6-(4,4-dimethylpent-2-ynyl)-4~{H}-pyrrolo[2,3-d][1,3]thiazole 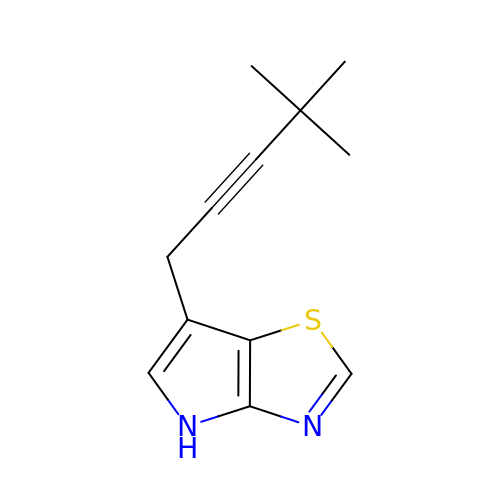| C12 H14 N2 S | JBYBLGDRQOCKRZ-UHFFFAOYSA-N> APSTDHLDYKDDDDKAAAKVFLCPGLLKGVYQSEHLFESDHQSGAWCKDPLQASDKIYYMPWTPYRTDTLTEYSSKDDFIAGRPTTTYKLPHRVDGTGFVVYDGALFFNKERTRNIVKFDLRTRIKSGEAIIANANYHDTSPYRWGGKSDIDLAVDENGLWVIYATEQNNGKIVISQLNPYTLRIEGTWDTAYDKRSASNAFMICGILYVVKSVYEDDDNEATGNKIDYIYNTDQSKDSLVDVPFPNSYQYIAAVDYNPRDNLLYVWNNYHVVKYSLDFGPLDSRSGPVHHGQVSYISPPIHLDSELERPPVRGILEVLFQ;> APSTDPKSCPSVCRCDAGFIYCNDRSLTSIPVGIPEDATTLYLQNNQINNVGIPSDLKNLLKVQRIYL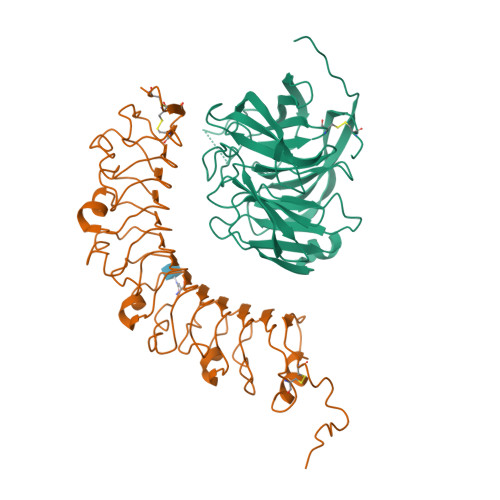YHNSLDEFPTNLPKYVKELHLQENNIRTITYDSLSKIPYLEELHLDDNSVSAVSIEEGAFRDSNYLRLLFLSRNHLSTIPGGLPRTIEELRLDDNRISTISSPSLHGLTSLKRLVLDGNLLNNHGLGDKVFFNLVNLTELSLVRNSLTAAPVNLPGTSLRKLYLQDNHINRVPPNAFSYLRQLYRLDMSNNNLSNLPQGIFDDLDNITQLILRNNPWYCGCKMKWVRDWLQSLPVKVNVRGLMCQAPEKVRGMAIKDLSAELFDCKDSGIVSTIQITTAIPNTAYPAQGQWPAPVTLEVLFQ>SVIKPDMKIKLRMEGAVNGHPFAIEGVGLGKPFEGKQSMDLKVKEGGPLPFAYDILTTVFSYGNRVFAKYPENIVDYFKQSFPEGYSWERSMNYEDGGICNATNDITLDGDCYIYEIRFDGVNFPANGPVMQKRTVKWEPSTEKLYVRDG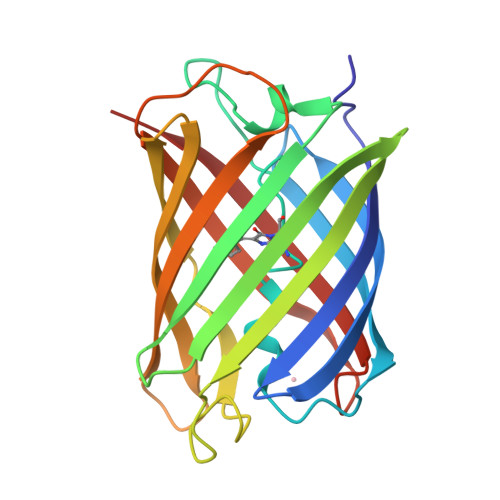VLKGDVNMALSLEGGGHYRCDFKTTYKAKKVVQLPDYHFVDHHIEIKSHDKDYSNVNLHEHAEAHSE[12x]>[2x]MAPFPEEVDVFTAPHW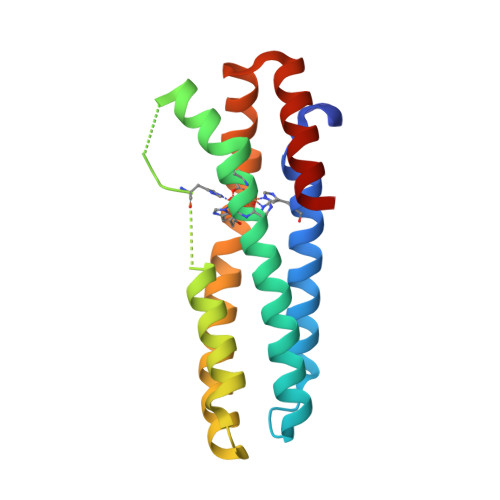RMKQLVGLYCDKLSKTNFSNNNDFRALLQSLYATFKEFKMHEQIENEYIIGLLQQRSQTIYNVHSDNKLSEMLSLFEKGLKNVKNEYEQLNYAKQLKERLEAFTRDFLPHMKEEEEVFQPMLMEYFTYEELKDIKKKVIAQHCSQ>HHHHHHSSGENLYFQGHMDDYSTRSNDNRIKLVPIAPSRGMIFDRNGTPLALNRTIYQLELMPEKIENLSATLNALRPIVDLTDDDIANFEKERKRSRRFTSIAVKTPLTEVQVARFAVNQFRFPGIEVKGYQRRFYPYGSALTHVIGYVSKINDKDVERLDKEGILPNY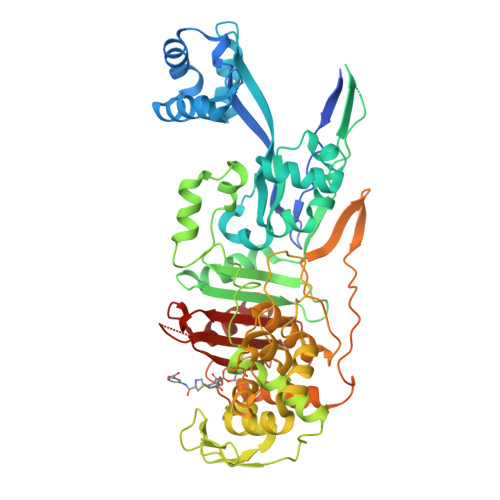AATHDIGKLGIERYYESTLHGKTGYEEVEVNNRGRVIRQLHEQPPQAGKDIYLTLDLSLQIYIEKLLSGSRAAVVVTDPRTGGILALVSNPSYDPNLFVDGISNKDYQGLLNDTNRPLINRATQGVYPPASTVKPYIAVSALSAGVITKNTSLFDPGWWQLPGSEKRYRDWKKWGHGRLNVTKALEESADTFFYQVAYDMGIDRLSSWMSKFGYGEYTGIDLSEERAGLMPTREWKQKRHKKPWYQGDTIPVGIGQGYWTATPIQMAKSLMTLINDGTVKTPHLLQSTRIDGVLVPYKQEDSTQIGSINSGYWEIAKDGMYGVANRPNGTGRKFFEGTPYKAAAKSGTAQVYSYETYNASKVAEHLRDHKLMVAFAPYENPTVSVAIILENGGAGPAVGTITRQILDHILLGD[2x]>APAAVDWREKGAVTPVKDQGQCGSCWAFSTIGNIEGQWQVAGNPLVSLSEQMLVSCDTIDFGCGGGLMDNAFNWIVNSNGGNVFTEASYPYVSGNGEQPQCQMNGHEIGAAITDHVDLPQDEDAIAAYLAENGPLAIAVDATSFMDYNGGILTSCTSEQLDHGVLLVGYNDASNPPYWIIKNSWS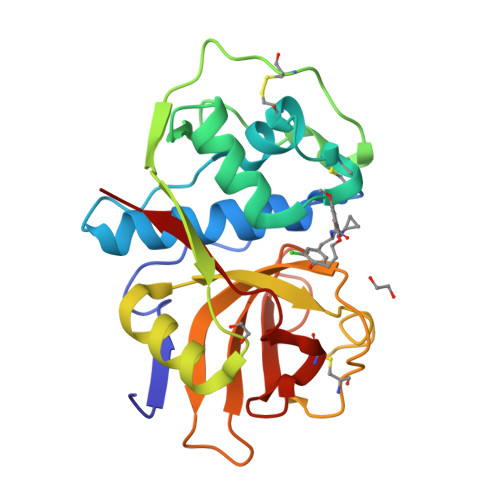NMWGEDGYIRIEKGTNQCLMNQAVSSAVVG[2x]> NLYFQGAMASIAIEYHSVVLGMERKVNVIYPDQSEIPKKDQGDKDIPVLYLLHGMGGNENSWQKRTAIERLLRHTNLIVVMPSTDLGWYTDTAYGLNYYRALSQELPQV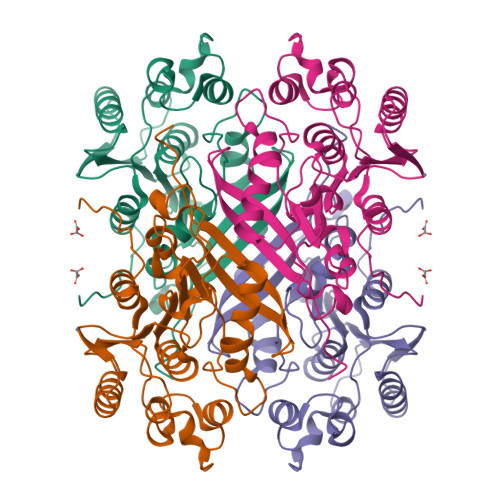LAAFFPNMTQKREKTFVAGLSMGGYGAFKWALKSNRFSYAASFSGALDFSPETNLEGNLGELAYWQGVFGQFEDPDLDKHYLKNMVAESDGKTKFYAWCGYEDFLFATNEKAIADFQAQGLDIDYHKGHGKHEWYYWNQQLEVLLEWLPINYQKEERLS>MKKIILTIGCPGSGKSTWAREFIAKNPGFYNINRDDYRQSIMAHEERDEYKYTKKKEGIVTGMQFDTAKSILYGGDSVKGVIISDTNLNPERRLAWETFAKEYGWKVEHKVFDVPWTELVKRNSKRGTKAVPIDVLRSMYKSMREYLGLPVYNGTPGKPKAVIFDVDGTL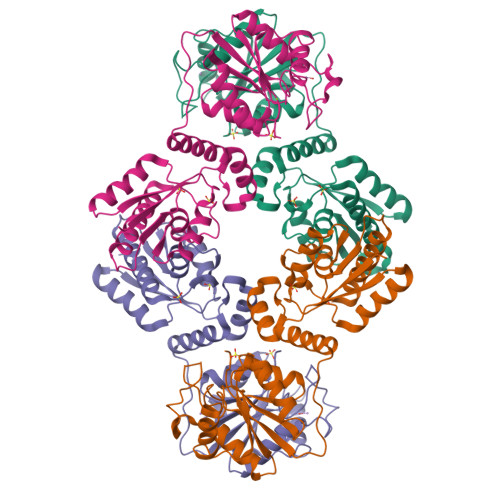AKMNGRGPYDLEKCDTDVINPMVVELSKMYALMGYQIVVVSGRESGTKEDPTKYYRMTRKWVEDIAGVPLVMQCQREQGDTRKDDVVKEEIFWKHIAPHFDVKLAIDDRTQVVEMWRRIGVECWQVASGDF[12x]Phorbol 12,13-dibutyrate | C28 H40 O8 | 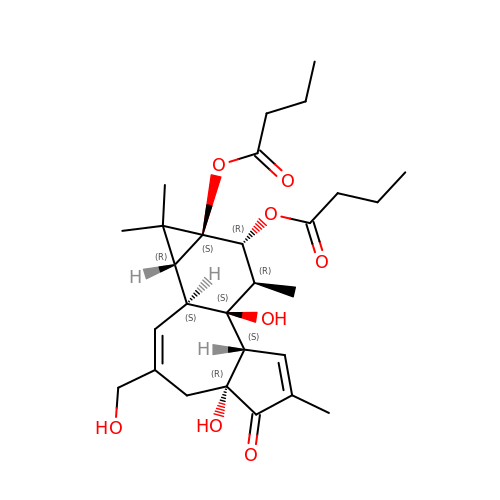BQJRUJTZSGYBEZ-YVQNUNKESA-N>MSLSMSKLEKLLKERGPIKKIGVLGMGYVGIPAAVLFADAPCFEKVLGFQRNSKSSGYKIEMLNRGESPLKGEEPGLEELIGKVVKAGKFECTPDFSRISELDAVTLAIQTPFANPKDLEPDFSALIDGIRNVGKYLKPGMLVVLESTITPGTTEGMAKQILEEESGLKAGEDFALAHAPERVMVGRLLKNIREHDRIVGGIDEASTKRAVELYSPVLTVGQVIPMSATAAEVTKTAENTFRDLQIAAINQLALYCEAMGINVYDVRTGVDSLKGEGITRAVLWPGAGVGGHCLTKDTYHLERGVKIGRGELDYPEGADSIYVLARKVNDFMPAHMYNLTVAALERLGKKMDGSKVAMLGWAFIKDSDDARNTPSEPYRDLCLKAGASVMVHDPYVVNYPGVEISDNLEEVVRNADAIVVLAGHSAYSSLKADWAKKVSAKANPVIIDGRNVIEPDE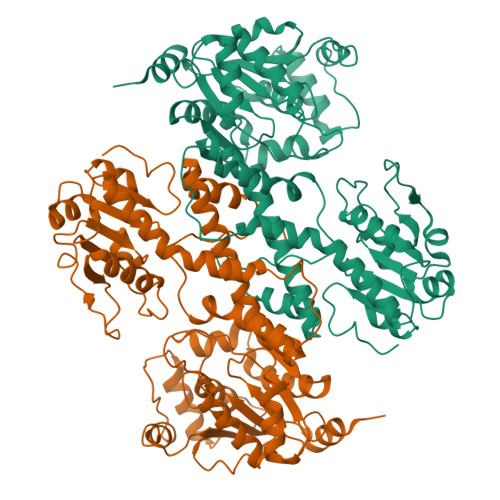FIGKGFVYKGIGREGHHHHHH[2x]>[4x]MAHHHHHHSSGLEVLFQGPGHKKKLEGKVAIVTGGASGIGETAARIFADHGARAVVIADIQSELGRMVAESIGAKRCSYVQCDIADEEQVKSAVEWTATTYGGL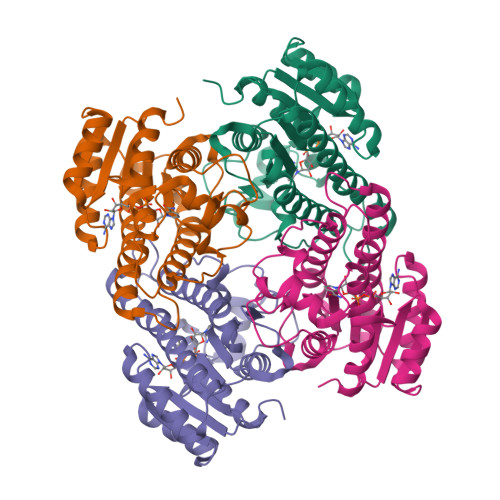DVMFCNAGIMSHSDSGQTVMELDMSKFDEVMRVNTRGTAACVKQAARKMVELGTRGGAIICTSSPLATRGGHVDTDYVMSKHAVLGLVRSASMQLGAHGIRVNSVSPMAVLTPLTRRMGLATPADVENALGRFTSLKGVALTAEHVAEAAAFLASDEAAFITGHDLVVDGGLLCLPFAAHS> MEDTMTMPSHAQLKAYFEEARDANEEYRKEAFIDRDYFDGHQWTEEELQKLEARKQPATYFNEVKLSIRGLVGVFEQGDSDPRAWPRNPQDEDSADIATKALRYVKDYSEWSDERSRAALNYFVEGTCAAIVGVDENGRPEIEPIRFEEFFHDPRSRELDFSDARFKGVAKWRFADEVGMEYGIKGEIDGALDGDSEGLSIGGDTFGDRPDGKISSWIDSKLRRVFVVEMYVRWNGVWIRALFWGRGILEMSVSAYLDRNGKPTCPIEARSCYIDRENRRYGEV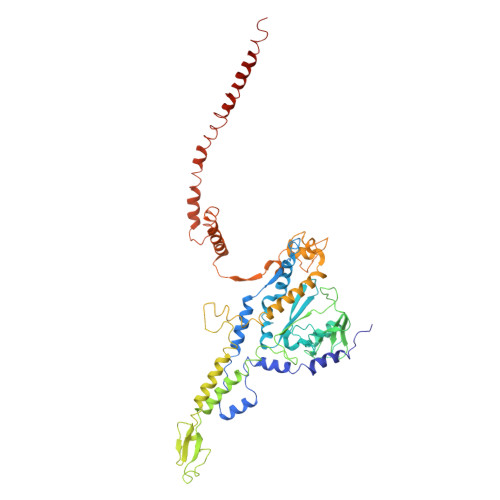RDLRSPQDAINKRESKLLHMLNNRQAIATNPEYAYNSDAEMVRKEMSKPDGIIPPGWQPASMTDLANGQFALLSSAREFIQRIGQNPSVLAAQSASASGRAQLARQQAGMVDSAMALNGLRRFELAVYRQAWLRCRQFWKAPDYIRVTDDEGAPQFVGINQPIKGPPQPVLNEMGQVVIAEPILGYENALAELDVDINIDAVPDTANLAQEQFLQLTELARLYGPQEVPFDDLLELSSMPEKTKLIAKRRERSEQMAQVQAQQGQMQEQIAMQGAMAEIENTQADTAYLAARAQNEMLKPQIEAFKAGFGAA>[2x]MSKKTIVSMAVIRRLPRYHRYLEELLKNDVKRISSRELSEKMGVTASQIRQDLNNFGGFGQQGYGYNVEELY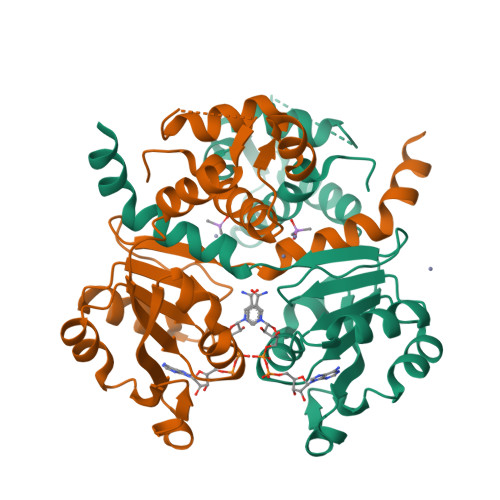NNLTKILGLDKTYNTIIIGAGNLGQAIANYTSFEKSGFNLKGIFDINPRLFGLKIRDVEVMDVETVEDFIARNKIDIGILCIPKDNAQYTADRLVRAGIKAIWNFLPIDLKVPDDVILENVHLSDSLFTVSYRLNEEELFKKLKGETAKIDG> STTEVVMENVTAFWEEGFGELLEKAKQNNN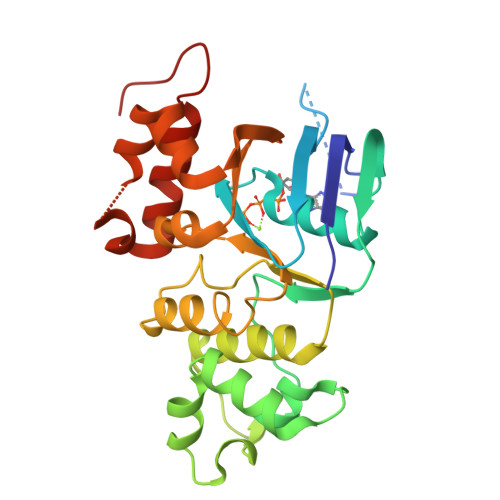NRKTSNGDDSLSFSNLSLLGTPVLKDINFKIERGQLLAVAGSTGAGKTSLLMMIMGELEPSEGKIKHSGRISFCSQFSWIMPGTIKENIIFGVSYDEYRYRSVIKACQLEEDISKFAEKDNIVLGEGGITLSEGQQAKISLARAVYKDADLYLLDSPFGYLDVLTEKEIFESCVCKLMANKTRILVTSKMEHLKKADKILILHEGSSYFYGTFSELQNLQPDFSSKLMGCDSFDQFSAERRNSILTETLRRFSLEGDAPVS>[4x]GPLGSMEKNMRPYTVLWADDEIDLLKPHILFLEQKGYQVTPVLSGNDAIEAVQNNDFDIVFLDENMPGIGGLDALQKIKELKPYTPVVMITKSEEEHIMTQAIGGKIADY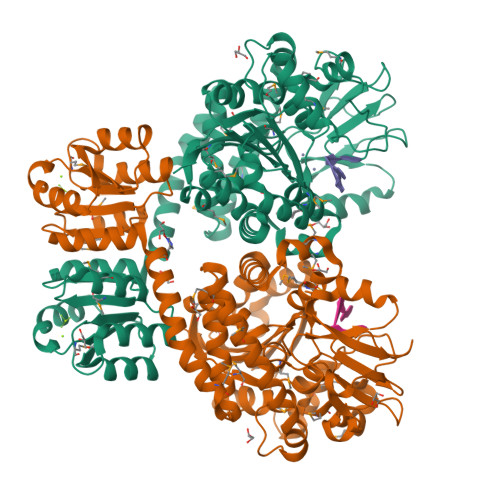LIKPVNPNQLLLSLKKNLQQHSIISETTNTNYRQEFVQLGTQMSGKLSFEEWKELYRRIVFWEIELEQADRQMGELLEMQKQEANRLFARFVTQNYREWIAKPDTRPTMSPDLFKQKVFPLLDNGEKVFFILIDNFRQDQWESVKSMLSEFYTFEEDMYLSILPTAAQYARNAIFSGLMPLQIEKMFPDLWVDEESEEGKNLNEEPMIRTLIERYRKHYSFSYNKVYETKFGERLLGQIRSLSQNQLNVIVLNFVDMMSHARTDSKMIRELASNEAAYRSLTKSWFKHSTTYNLFRSIAEMGYKVVLTTDHGTIQVKNPVKVIGDRSTNTNLRYKIGKNLDYNPKEVFEIKDPASVGLPHNNLSDKFIFTKEDDFFAYPNNYNYYVQYYRNTFQHGGISLEEMLVPVITMQPK Multi-subunit SMC complexes control chromosome superstructure and promote chromosome disjunction, conceivably by actively translocating along DNA double helices. SMC subunits comprise an ABC ATPase “head” and a “hinge” dimerization domain connected by a 49 nm coiled-coil “arm. The heads undergo ATP-dependent engagement and disengagement to drive SMC action on the chromosome. Here, we elucidate the architecture of prokaryotic Smc dimers by high-throughput cysteine cross-linking and crystallography.

To understand how the Smc joint connects to the Smc head at the end of the Smc rod, we next solved the structure of PySmcHd-CC80, a Pyrococcus yayanosii Smc head attached to a long coiled coil that includes the Smc joint. Based on sequence and structure comparison, we mapped the Bs Smc cross-linking efficiencies onto PySmcHd-CC80 (right). Remarkably, these residues form a straight line on the surface of the molecule, the presumptive 2-fold symmetry axis of the Smc rod. We then manually aligned two PySmcHd-CC80 molecules aiming to minimize the distance between all cross-linkable residues. The resulting Smc rod fragment shows an intimate association between the two PySmcHd-CC80 monomers with little steric clashes. While the Cα-Cα distance is relatively large (>20 Å) for some residues, indicating that the model of the PySmcHd-CC80 dimer is not a perfect representation of the structure of native Bs Smc-ScpAB, overall there is excellent alignment of most pairs of experimentally identified Bs Smc axial residues.

> MPYIEKLELKGFKSYGNRKVVIPFSKGFTAIVGANGSGKSNIGDAILFVLGGLSAKAMRATRISDLIFAGSKGEPPAKYAEVAIYFNNEDRGFPIDEDEVVIKRRVYPDGRSAYWLNGRRATRSEILDLLSAAMISPEGYNLVLQGDITKFIKMSPLERRQLIDEISGIAEYDAKKEKALEELKQAEENLARVDLLIKEVKKQLDKLEKERNDALRYLDLKERLERARVALLLGEIKRLESMIDEGERKRAEIESGGSENTIKVKSAQLRIQLEEKRRELKHFDAALIRSVKEVSLDLEVLRKEIEDMEAEIKALEPVNMKAIEDFEVVERRYLELKSKREKLEAEKESIIEFINEIEKEKKNVFMRTLEAIAKNFSELFAKLSPGGSARLILENPEDPFSGGLEIEAKPAGKDVKRIEAMSGGEKALTALAFIFAIQRFKPAPFYLFDEIDAHLDDANVKRVADLIKESSRESQFIVITLRDVMMANADKIIGVSMRDGVSRVVSLSLEKAMKILEEAKKRNEATIGGVDAGSSSRPGL The mitochondrial F1Fo-ATP synthase produces most of the ATP in the cell by rotary catalysis and plays a crucial role in severe human neurodegenerative disorders (Kucharczyk et al., 2009). The proton motive force (pmf) across the inner membrane drives the c-ring rotor in the membrane-embedded Fo subcomplex, generating the torque that powers a sequence of conformational changes in the membrane-extrinsic F1 subcomplex, resulting in ATP generation (Abrahams et al., 1994, Boyer, 1997, Noji et al., 1997). The Fo subcomplex is connected to F1 by the central stalk, which transmits torque to the catalytic head, and the peripheral stalk, which acts as a stator to prevent idle rotation of the F1 head with the c-ring. We determined the structure of a complete, dimeric F1Fo-ATP synthase from yeast Yarrowia lipolytica mitochondria by a combination of cryo-EM and X-ray crystallography.

Crystals of the YLF1c10 subcomplex were obtained from the 1YLF1Fo complex. Whereas previous crystallographic studies of similar complexes (Giraud et al., 2012, Pagadala et al., 2011, Stock et al., 1999) used an excess of nucleotide substrates or inhibitors to trap functional states, we crystallized YLF1c10 without any such additives to ensure similar conditions for crystallography and cryo-EM. The 3.5 Å X-ray structure of YLF1c10 reveals that all three non-catalytic α subunits bind Mg·ATP in their nucleotide sites. Of the three catalytic β subunits, one is empty (βE), while both the βDP and βTP sites (Abrahams et al., 1994) contain Mg·ADP. A detailed comparison of the YLF1c10 crystal structure to the bovine (Abrahams et al., 1994) and Saccharomyces cerevisiae (Kabaleeswaran et al., 2006) F1 and F1c10 complexes reveals that the three conformational states of the corresponding α/β heterodimers are very similar in the two yeast species, with root-mean-square deviation (RMSD) values below 1.7 Å, while nucleotide binding and C-terminal regions of the bovine β subunits differ. In YLF1c10 both the βE and the βDP site are more open than in the bovine complex, while their βTP sites are similar. Aligning the γ subunits in all F1 X-ray structures and comparing the relative positions of the conserved P loop in the βDP subunit, we find that the YLF1c10 P loop is shifted to a position that, in bovine F1 (Rees et al., 2012), would indicate a post-hydrolysis or pre-product release state. The post-hydrolysis position of the γ subunit in YLF1c10 agrees with the presence of bound Mg·ADP in the catalytic βDP and βTP sites. Since YLF1c10 was crystallized without added nucleotides, the ADP originates from ATP hydrolysis during isolation or crystallization (Abrahams et al., 1996, Gledhill et al., 2007). We found the inhibitor protein IF1 bound to one of the three different rotational F1 states in the cryo-EM maps, but not in the YLF1c10 X-ray structure, indicating that it was lost during crystallization.

>[3x]MFKNALRRAGVAAPRISRVAQRGYAEAKATPTEVTSILEERIRGVSGEANLNETGRVLSVGDGIARVFGLNNIQAEELVEFASGVKGMALNLEAGQVGIVLFGSDRLVKEGETVKRSGSIVDVPVGPALLGRVVDALGNPIDGKGPIETEFRIRAQVKAPGILPRTSVNEPMQTGLKAVDALVPIGRGQRELIIGDRQTGKTQIAIDTILNQKRWNYGQDEKKKLYCVYVAVGQKRSTVAQLVQTLEHHDALKYSIIVAATASEAAPLQYLAPFTGTAMGEWFRDNGKGALIVFDDLSKQAVAYRQMSLLLRRPPGREAYPGDVFYLHSRLLERAAKMNEREGGGSLTALPIIETQGGDVSAYIPTNVISITDGQIFLEAELFYKGIRPAINVGLSVSRVGSAAQVKAMKQVAGSLKLFLAQYREVAAFAQFGSDLDASTKQTLTRGERLTLLLKQKQASPMSSEEMVPLIYAGVNGYIDNIPVKQVEKFEAEFVSYLHANESDLLKDIAATGELSKENLEKLKSITENFVGSFAK;>MVLPRLIPRLSRSAFKVAQANNRVFNAPFRGMASSAGVGSGKIRTVIGAVVDVQFEQDNLPAILNALTIDRGEGNKLVLEVAQHLGENTVRTIAMDGTEGLVRGTSVADTGAPITIPVGRGTLGRIINVCGEPIDERGPIEATKFLPIHADPPTFAEQSTTAEVLETGIKVVDLLAPYARGGKIGLFGGAGVGKTVFIQELINNIAKAHGGFSVFCGVGERTREGNDLYREMKETGVINLEGESKVTLVFGQMNEPPGARARVALTGLTIAEYFRDEEGQDVLLFVDNIFRFTQAGSEVSALLGRIPSAVGYQPTLATDMGALQERITTTQKGSVTSVQAVYVPADDLTDPAPATTFAHLDATTVLSRGISELGIYPAVDPLDSKSRLLDIDVVGQEHYDVASNVQQTLQAYKSLQDIIAILGMDELSEQDKLTVERARKIQRFLSQPFTVAEVFTGIEGRLVSLKDTVRSFKEILDGKHDALPEAAFYMVGGIEEVVAKAEKLAAESK[3x];> MFALRTAARPAARSVGATRNYATLREIEMRLKSIKNIEKITNTMKIVASTKLGKAQRAMATSKVYNEASEKVFENSETAVPENIEKRLWVVVSSDKGLCGSIHSQLARTVRRKLLDFESGEKLIDIVAVGEKIKAQLGRSNPEQMRLSFGGTGKEAPTFEEAAHIADEILALDTQYDDIEIVYNKVLSGISFEPIMKESYSAKAIEDAPKFGQYELEDDVVKNLADFSLANTIYAAMAEGHAAEISARRNAMDNASKNASDMINKYSILYNRTRQAVITNELVDIITGASSLE;> MSDHTRSQNWTNLILTQSIYNQKEVTQVNIPSTAGELGILANHVPTIQQLKPGVVEVIETNGETKSYFISGGFATVQPDSELSVNSIEAFQAEDFSPEAIKSLTAEAQKNAQSADEAVAAEAEIELEVLEALAHFAK;>[10x]MQLVLAGKYIGAGLASIGLVGAGIGIAIVFAALINGVSRNPALKGQLFTYSILGFALSEATGLFALMIAFLLLYAV N-benzyl-4-[(2R)-pyrrolidin-2-ylmethoxy]aniline | C18 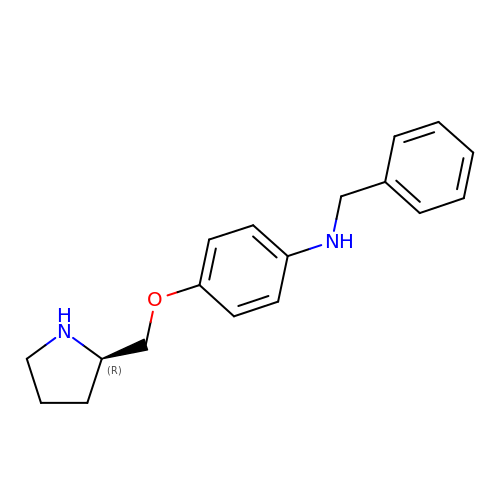H22 N2 O | HITMFLNAOQIZSN-QGZVFWFLSA-N> MPSLMSFGSCQWIDQGRFSRSLYRNFKTFKLHEMHGLCMPNLLLNPDIHGDRIIFVCCDDLWEHDLKSGSTRKIVSNLGVINNARFFPDGRKIAIRVMRGSSLNTADLYFYNGENGEIKRITYFSGKSTGRRMFTDVAGFDPDGNLIISTDAMQPFSSMTCLYRVENDGINFVPLNLGPATHILFADGRRVIGRNTFELPHWKGYRGGTRGKIWIEVNSGAFKKIVDMSTHVSSPVIVGHRIYFITDIDGFGQIYSTDLDGKDLRKHTSFTDYYPRHLNTDGRRILFSKGGSIYIFNPDTEKIEKIEIGDLESPEDRIISIPSKFAEDFSPLDGDLIAFVSRGQAFIQDVSGTYVLKVPEPLRIRYVRRGGDTKVAFIHGTREGDFLGIYDYRTGKAEKFEENLGNVFAMGVDRNGKFAVVANDRFEIMTVDLETGKPTVIERSREAMITDFTISDNSRFIAYGFPLKHGETDGYVMQAIHVYDMEGRKIFAATTENSHDYAPAFDADSKNLYYLSYRSLDPSPDRVVLNFSFEVVSKPFVIPLIPGSPNPTKLVPRSMTSEAGEYDLNDMYKRSSPINVDPGDYRMIIPLESSILIYSVPVHGEFAAYYQGAPEKGVLLKYDVKTRKVTEVKNNLTDLRLSADRKTVMVRKDDGKIYTFPLEKPEDERTVETDKRPLVSSIHEEFLQMYDEAWKLARDNYWNEAVAKEISERIYEKYRNLVPLCKTRYDLSNVIVEMQGEYRTSHSYEMGGTFTDKDPFRSG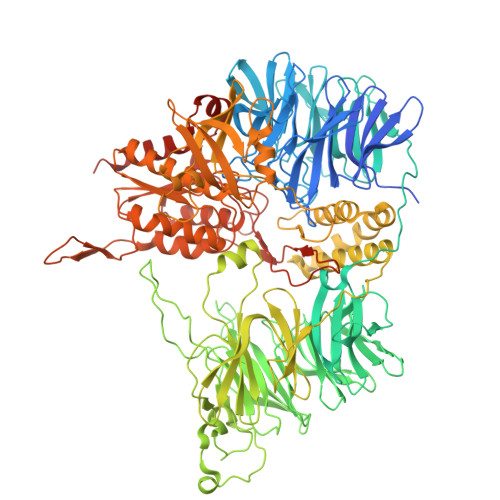RIACDFKLDGDHYVVAKAYAGDYSNEGEKSPIFEYGIDPTGYLIEDIDGETVGAGSNIYRVLSEKAGTSARIRLSGKGGDKRDLMIDILDDDRFIRYRSWVEANRRYVHERSKGTIGYIHIPDMGMMGLNEFYRLFINESSYQGLIVDVRFNGGGFVSQLIIEKLMNKRIGYDNPRRGTLSPYPTNSVRGKIIAITNEYAGSDGDIFSFSFKKLGLGKLIGTRTWGGVVGITPKRRLIDGTVLTQPEFAFWFRDAGFGVENYGVDPDVEIEYAPHDYLSGKDPQIDYAIDALIEELRNWNEELPQRPS>TQQNTPLADDTTLMSTTDLQGYITHANDTFVQVSGYTLQELQGQPHNMVRHPDMPKAVFADMWFTLKKGEPWSGIVKNRRKNGDHYWVRANVVPMVREGKISGYMSIRTRATDEEIAAVEPLYKALN[2x]

The primary energy sensor for motility in Escherichia coli is the dimeric transmembrane chemoreceptor Aer (aerotaxis receptor), which responds to changes in oxygen concentration indirectly by monitoring the metabolic load of reducing equivalents in the ETC. Aer is dimeric and composed of a cytoplasmic N-terminal PAS (Per–Arnt–Sim; named for the representative proteins: Period, Aryl hydrocarbon receptor nuclear translocator protein and Single-minded) domain, a helical transmembrane domain, a cytoplasmic HAMP (histidine kinases, adenylate cyclases, methyl-accepting chemotaxis proteins [MCPs], and phosphatases) domain, and a C-terminal coiled-coil kinase control domain (KCD) with high homology to those of MCPs. The sensory module of Aer is the intracellular PAS domain that binds a redox-sensitive flavin adenine dinucleotide (FAD) prosthetic group. The flavin undergoes changes in redox state that trigger conformational transitions within the PAS domain that propagate to the KCD to transduce Aer signaling events.

Here, we report the structure and biophysical characterization of the Aer PAS domain, making use of the triple variant that combines all three flavin-stabilizing residue substitutions (S28G, A65V, and A99V); hereafter, called, Aer-PAS-GVV. The structure of Aer-PAS-GVV was determined to a 2.4 Å resolution by using a molecular replacement probe derived from AlphaFold; the structure contains two molecules within the asymmetric unit. The PAS core of Aer-PAS-GVV forms the FAD-binding pocket and consists of five antiparallel β-strands (Aβ, Bβ, Gβ, Hβ, and Iβ) and several peripheral α-helices (Cα, Dα, Eα, and Fα). Flanking the PAS core are an N-terminal coil that extends across a cleft in the β-sheet to the Gβ–Hβ loop and a C-terminal helix that sits above Gβ, Hβ, and Fα. Of the two Aer-PAS-GVV molecules in the asymmetric unit; chain B is considerably more disordered and has higher B-factors than chain A. The three substitutions that stabilize the Aer PAS domain are in relatively close proximity to the flavin. S28G is on a loop between Aβ and Bβ, with its carbonyl oxygen hydrogen bonding with the amide nitrogen of H53. The Ala to Val substitution appears to fill in a cavity otherwise produced by M61, Y130, V83, and L133. The A99V substitution increases hydrophobic interactions to the dimethylbenzene ring of FAD that likely serve to increase cofactor stability in the pocket. The side chain amide nitrogen and carbonyl oxygen of residue N85 hydrogen bonds with the O4 and N3 atoms of the FAD, respectively, and the imidazole ring of H53 forms π–π stacking interactions with the FAD pyrazine ring.> MAHHHHHHVGTGDWRTATSLYEFSAPDIDGNMVDLSKYRGH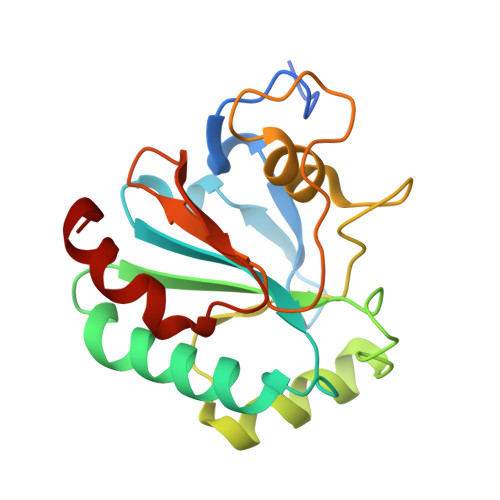TVIVTNVASQCGKTEVNYKQLVELHERYAERGLRILAFPCNQFGKQEPGSNAEIKEFMARYNVKFDMFAKIDVNGDSAHPLWKWLREQPNGKGIGGNAIKWNFTKFLIDKEGKVVKRYGPMDEPKVIEADLPKYF>[3x]GPHMSTEKAPAALGPYSQAIKANNLVFLSGVLGLIPETGKFVSESVEDQTEQVLKNMGEILKASGADYSSVVKTTIMLADLADFKTVNEIYAKYFPAPSPARSTYQVAALPLNAKIEIECIATL

Arabidopsis thaliana RidA (AtRidA) is targeted to chloroplasts. By converting the reactive enamine/imines to harmless 2-oxoacids, RidA preempts damage to BCAT3 and ensures that the isoleucine biosynthesis can proceed. In this study, we determined the crystal structures of apo-AtRidA and its complex with pyruvate, and analyzed its structural basis for ligand recognition. The RidA domain retains the basic overall fold, and also preserves the homotrimeric structure with the characteristic interfacial clefts.

Therefore we tried both 2-oxoacid products for cocrystallization studies, and we obtained the complex structure of AtRidA bound by pyruvate. The structure was obtained by soaking the crystals of the apoprotein with 20 mM pyruvate for 1 hour, and the resulting crystals diffracted to 2.3 Å. The crystals did not appear to have decayed, but the crystal space group became P1. After structure determination, we found that there were three monomers present in the asymmetric unit. The three monomers within the asymmetric unit form the trimeric barrel, which is almost identical to that formed by the apoprotein, with an RMSD of only 0.27 Å. Pyruvate binds to the interfacial cleft formed by two subunits, but makes specific hydrogen bonds with only one subunit. The carboxylate group of pyruvate forms the salt bridge with the NH2 and NE atoms of the guanidino group of conserved R165, while accepting another from the OG atom of T167. Additionally, O3 of the carbonyl group receives another hydrogen bond from the backbone of T167. Aside from these polar contacts, the ligand is located at the active site formed by F147, L95 and P174. Additionally, the terminal carboxylate of E180 from the neighboring subunit is only 3.26 Å from the 2-carbonyl group, and hence it is very likely to play a role in the recognition of the intermediates.>SNAMPVRVIVDSSACLPTHVAEDLDITVINLHVMNNGEERSTSGLSSLELAASYARQLERGGDDGVLALHISKELSSTWSAAVTAAAVFDDDSVRVVDTSSLGMAVGAAAMAAARM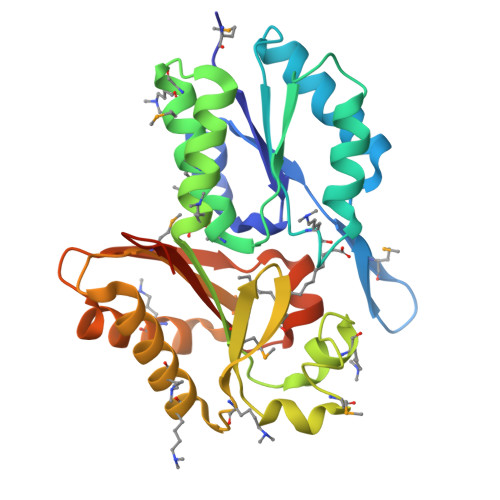AKDGASLQECYDIAVDTLKRSETWIYLHRIDEIWKSGRISTATAMVSTALATRPIMRFNGGRMEIAAKTRTQSKAFAKLVELAQIRADGEPVFIAIGQNEAREAAKQLEELLRNALPEGSSFMSVDIDPTLAVHSGPGAVSVSAVFANQAPELSTGKAGAK[3x]> GSEELQGLKDDVEKLTADAELQRLKNERHEEAELERLKSERHDHDKKEAERKALEDKLADKQEHLNGALRYI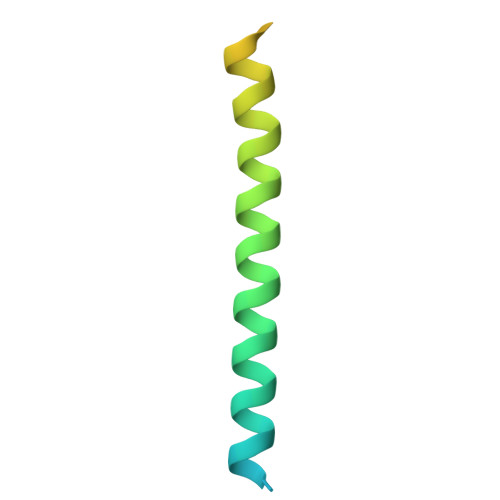NEKEA>[4x]MDKLREKINAARAETDEAVARAEAAEAKLKEVELQLSLKEQEYESLSRKSEAAESQLEELEEETKQLRLKADNEDIQKTEAEQLSRKVELLEEELETNDKLLRETTEKMRQTDVKAEHFERRVQSLERERDDMEQKLEEMTDKYTKVKAELDEVHQALEDL

Cables formed by head-to-tail polymerization of tropomyosin, localized along the length of sarcomeric and cytoskeletal actin filaments, play a key role in regulating a wide range of motile and contractile processes. Here, we present high–resolution structures of cables formed by acetylated and unacetylated Schizosaccharomyces pombe tropomyosin ortholog TpmCdc8. All homodimer conformers are approximately 230 Å in length and exhibit head–to–tail interactions, where the N–termini of one homodimer contact the C–termini of an adjacent homodimer. Each of the conformers that make up the TpmCdc8 cables consists of two α-helices that are wrapped around each other, forming a left-handed coiled–coil structure.

The SeMet–derivatized unacetylated TpmCdc8 crystallized in space group P21 and diffracted to 2.4 Å resolution. The structure was solved by Single wavelength Anomalous Dispersion (SAD) phasing. Here, the asymmetric unit contains two TpmCdc8 homodimers of different conformations (conf-U2 and conf-U3). Conf-U1 and conf-U2 have a straight coiled–coil structure, whereas conf-U3 contains a central 24° kink. Most likely, these three different conformers represent trapped states in response to different elastic and torsional loads. The largest difference between chain A and chain B of a given conformer is 9.0 Å for conf-U3, which in this case is primarily attributable to its central kink. The greatest similarity is shared by conf-U1 chain B and conf-U2 chain A with an rmsd of 1.7 Å. As predicted by an analysis of the B-factors of the conformer structures, conf A1 showed a narrow ensemble distribution, while those for conf-U1, conf-U2 and conf-U3 were much wider indicating increased flexibility of their overlap junctions. The interaction energies of the conformers are −50.5 kcal/mol for conf-A1, −27.2 kcal/mol for conf-U1, −55.0 kcal/mol for conf-U2 and −40.3 kcal/mol for conf-U3.>TPYMVQPEYRIYEMNKRLQSRTEDSDNLWWDAFATEFFEDDATLTLSFCLEDGPKRYTIGRTQIPRYFSTVFEGGVTDLYYILKHSKESYHNSSITVDCDQCAMVTQHGKPMFTKVCTEGRLILEFTFDDLMRIKTWHFTIRQYRELVPRSILAMHAQDPQVLDQLSK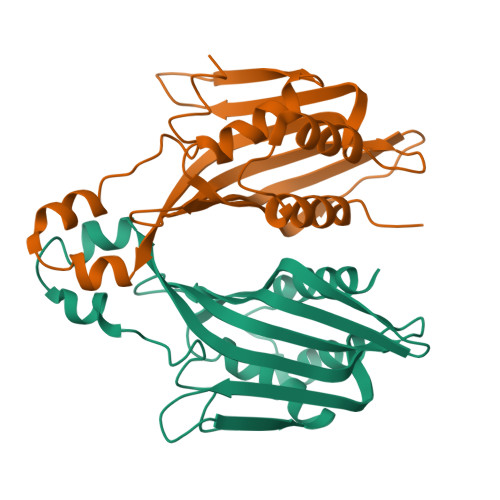NITRMGLTNFTLNYLR[2x]> MFRRIISNGALLSTQTQRWQDLSKFACLRASLNKESEKAFQELAKKNNVSPQELVELSKIVSMNLDVLKQNINSEQFLLEKESTLKRYRQSSIGTRGHLQTVNEAVNTKYPTLAEGLGQVAGYKEAYQALREIFVHPSISVNNLRQGSYGQQFAVDFRTRADEYVKALLKDHSSNPQAVQTIQEIQHTLHQIIKNYEQNPASIYARILT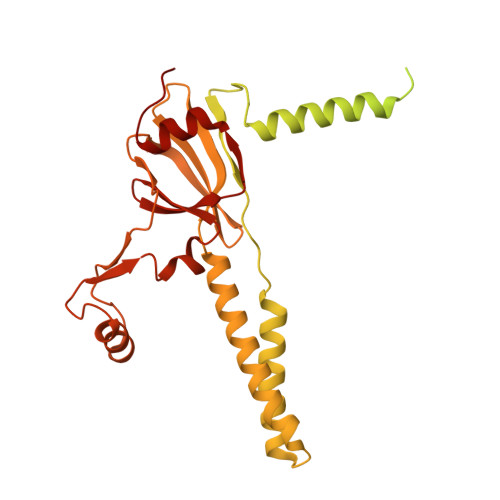VLQTRGVNTLPVSKTADQKAVATIQKTSTPSLTIDQLTVPVQERVQTQTVFDAELAFIKEANEMIQQNTGNLPWDGGKKKIFQGQANKYLETPYYLLAALSGLGLLYFLYSGDAKYKTLVLTPVVGIAAFVLLRRNQILNRVPTLTELFLHKDGKFVDAVVSVNGQLISKNDIPVSTLKLYRGDHTVKVNLNDFEDASAKKFLAQQSGQEGVINVHFSKLRNLAARNGQVLNLGDTEVVVPFENQANRIILKQIFKGVEVLPSS2-{[[(1S)-1-AMINO-2-CARBOXYETHYL](DIHYDROXY)PHOSPHORANYL]METHYL}-4-METHYLPENTANOIC ACID | C10 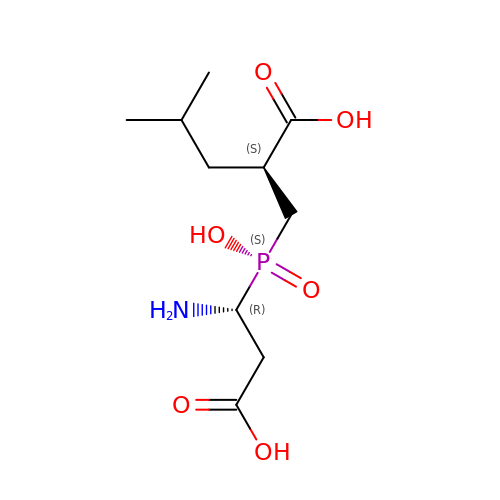H20 N O6 P | UCHSLOWIDRXYFJ-HTQZYQBOSA-N> ARENEMDENLEQVSGIIGNLRHMALDMGN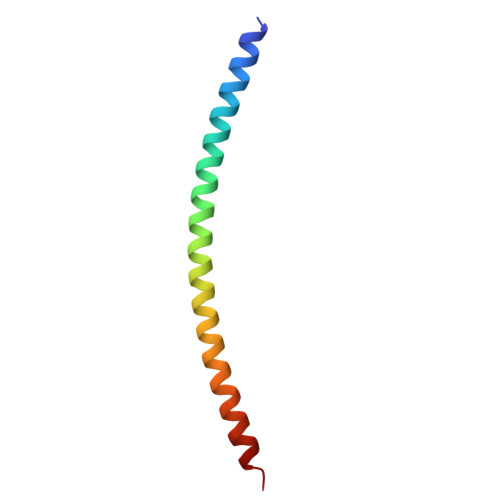EIDTQNRQIDRIMEKADSNKTRIDEANQRATKMLG>SNAMVQAQTRDQIVAAADELFYRQGFAQTSFVDISAAVGISRGNFYYHFKTKDEILAEVIRLRLARTAQMLADWQGTGDSPRARIASFIDLMIMNRAKITRYGCPVGSLCTELSKLDHAAQGQANGLFTLFRDWLQRQFAEAGCTTEAPALAMHLLARSQGAATLAQSFHDEGFLRSEVADMHR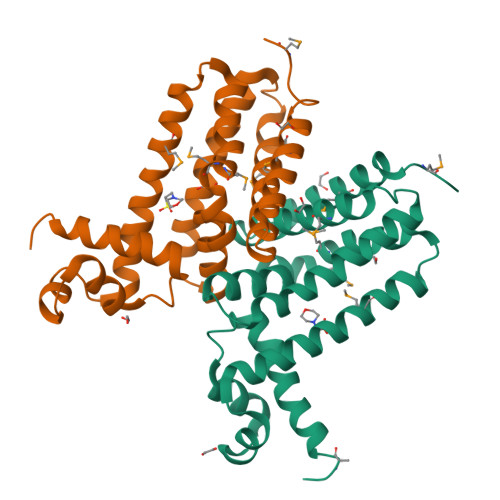WLDNTLPMTT[8x]> ACDVSIEGNDSMQFNTKSIVVDKTCKEFTINLKHTGKLPKAAMGHNVVVSKKSDESAVATDGMKAGLNND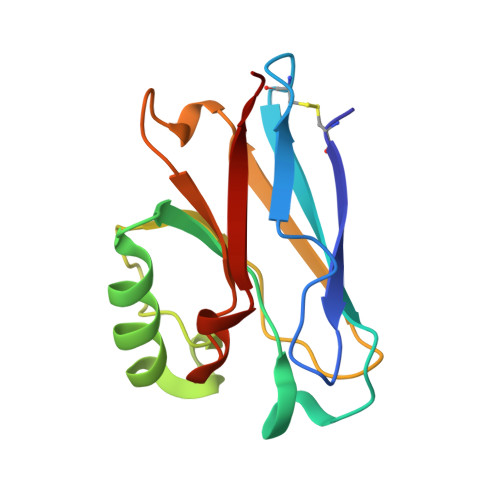YVKAGDERVIAHTSVIGGGETDSVTFDVSKLKEGEDYAFFCSFPGHWSIMKGTIELGS> IFGIDDLIFGLLFVGFVAGGVAGGYFWGRSNGGGGGASVSSTQAGFDKIGKDIQQLRNDTNAAIEGFNGRIAHDEQAIKNLAKEIEDARAEALVGELGIIRSLIVANISMNLKESLYELANQITKRGGG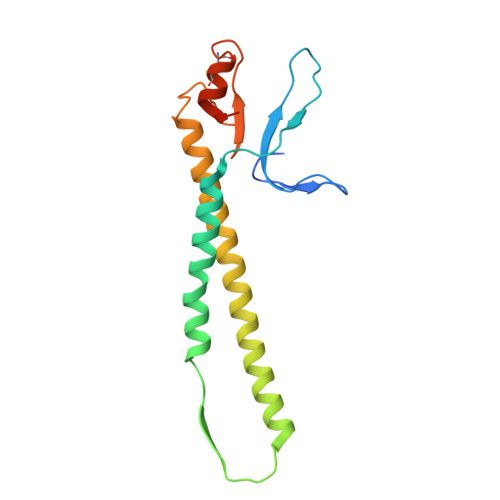IAQEAGPGCWYVDSENCDASCKEYIFNFNGSATVPTL>ATAAEIAALPRQKVELVDPPFVHAHSQVAEGGPKVVEFTMVIEEKKIVIDDAGTEVHAMAFNGTVPGPLMVVHQDDYLELTLINPETNTLMHNIDFHAATGALGGGGLTEINPGEKTILRFKATKPGVFVYHCAPPGMVPWHVVSGMNGAIMVLPREGLHDGKGKALTYDKIYYVGEQDFYVPRDENGKYKKYEAP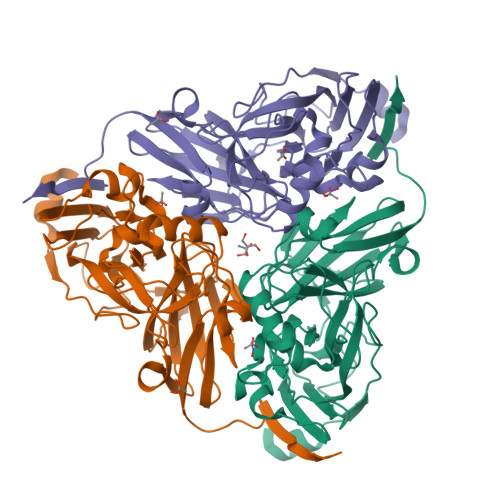GDAYEDTVKVMRTLTPTHVVFNGAVGALTGDKAMTAAVGEKVLIVHSQANRDTRPHLIGGHGDYVWATGKFNTPPDVDQETWFIPGGAAGAAFYTFQQPGIYAYVNHNLIEAFELGAAAHFKVTGEWNDDLMTSVLAPSGTIEGR[3x]>MVQTSFEHHHHHHSAGENLYFQGAQISMRLYSNRDRPNHLGPLALERLARVDDVVAQPARQPEDGFAASEDSLLGDVEEYARLFTRFLDGPVAPLGDAIPDDPARRAENLKASAYFLDASMVGICRLDPDDRAGDCDPSHTHALVFAVQFGREPEAGEAGAEWIRGTNAARTDMRCAEIAAILSGYVRWMGFPARGHFSGDAQVDLARLAVRAGLARVVDGVLVAPFLRRGFRLGVVTTGYALAADRPLAPEGDLGETAPEVMLGIDGTRPGWEDAEEEKRPLHMGRYPMETIRRVDEPTTLVVRQEIQRVAKRGDFFKRAEAGDLGEKAKQEKKRFPMKHPLALGMQPLIQNMVPLQGTREKLAPTGKGGDLSDPGRNAEAIKALGYYLGADFVGICRAEPWMYYASDEVEGKPIEAYHDYAVVMLIDQGYETMEGASGDDWISASQSMRAYMRGAEIAGVMAAHCRRMGYSARSHSNAHSEVIHNPAILMAGLGEVSRIGDTLLNPFIGPRSKSIVFTTDLPMSVDRPIDFGLQDFCNQCRKCARECPCNAISFGDKVMFNGYEIWKADVEKCTKYRVTQMKGSACGRCMKMCPWNREDTVEGRRLAELSIKVPEARAAIIAMDDALQNGKRNLIKRWWFDLEVIDGVAGAPRMGTNERDLSPDRGDKIGANQKLAMYPPRLQPPPGTTLDAVLPVDRSGGLAEYAAAETPAAARARLKSS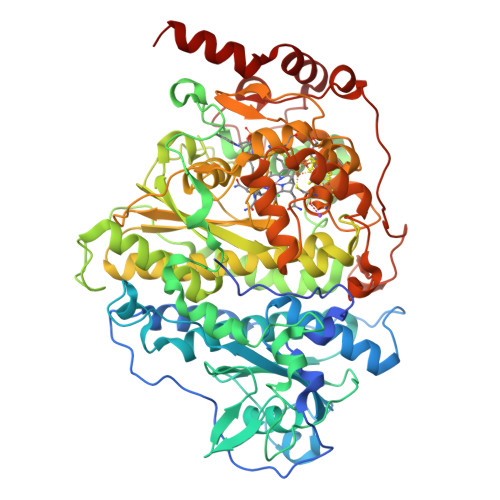AG[3x]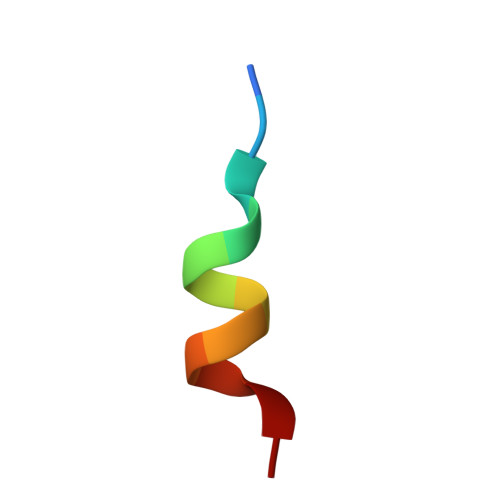> KHKILHRLLQDS> MASWSHPQFEKIEGRMSVTVPNDDWTLSSLSETFDDGTQTLQGELTLALDKLAKNPSNPQLLAEY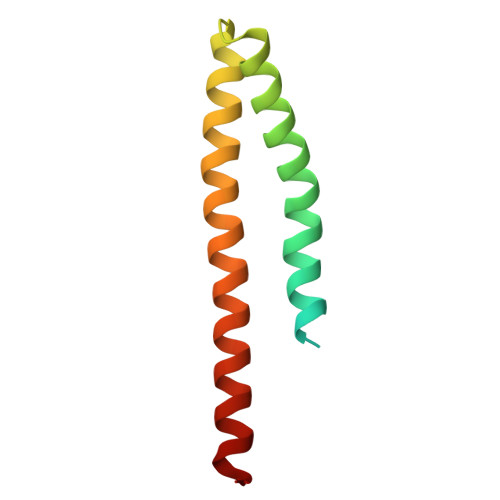QSKLSEYTLYRNAQSNTVKVIKDVDAAIIQNFR>MRSSKIRCPGAIRVGTLVTAFGCLPHVAFAAAREAPPVTPEVLVRLADIGTMSASETTPLLSLSPDGRYVAFQVRQADPVTNLNVFRMVVKATDGATDAIDVDVGGEYLFWTIPSWGYARNAPSGANLTIQPRWSPSGTHLAYLRQDQGRVRVWRASVKGEGASPVIEDAYDIEDVQWLDDNTLIYSGRPGFVEAEAEIEREGRRGWVYDERFHPLTGARPRVLEPISIVYQVLDLKTGTRRAATPTEVARLREKPDP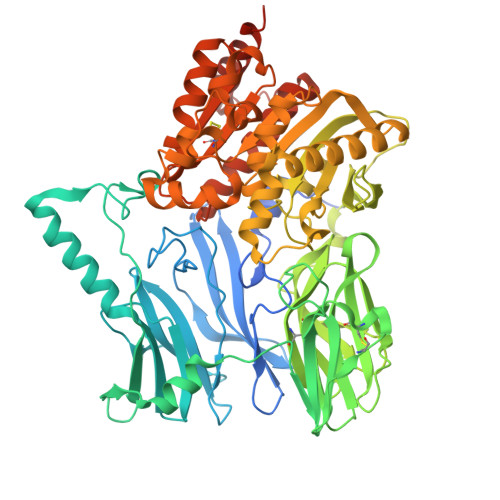LRAMVGRTTFSVSRTDPQNINAPTTLVARRGEGEPVRCDEEACQNITRMWGDETANVLYFLRREGWASNEMALYRMPADALKPVRIWHATGLLQGCERQAKRLICAQESALQPRRLVTLNLTSGQMSPLYDPNPDLSRYRLPKVERLTLRNRNGIEVFSDLVLPPDYQLGTRLPLVIVQYSSRGFLRGGTGDENPILPLATAGFAVLSFHSPRSEASYQRFTSPIAQSKAEYSNWRNRWNILHTLEDLIDDLDRRGVIDPARVGLTGLSDGATTVHFGLINSHRFAAAVTSSCCTDSFTASVMNGPRISGALKAYGIETDQADDGPFWAATSFVVNASRLDTPLLIQSADEEYLGALPGFTALQQARKPVELIIYPNEHHVKWQPAHRLAVYNRTIDWFRFWLMDQSDPAPDKAAQYDRWRALRALRQKSPSPTPAPGSRSHHHHHH[2x]>[2x]TRDQNGTWEMESNENFEGWMKALD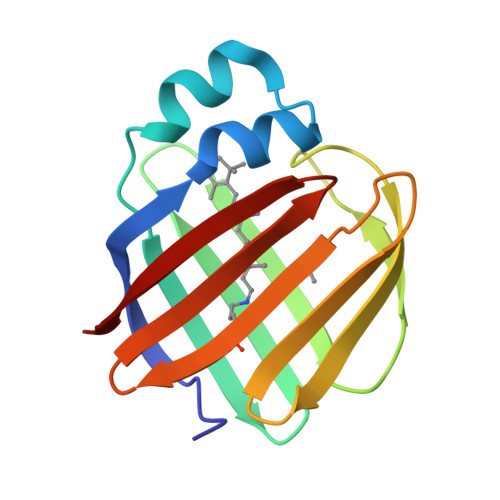IDFATRKIAVRLTQTLVIDQDGDNFKVKTTSTFWNYDVDFTVGVEFDEYTKSLDNRHVKALVTWEGDVLVCVQKGEKENRGWKKWIEGDKLYLELTCGDQVCRQVFKKK>HPICEVSKVASHLEVNCDKRNLTALPPDLPKDTTILHLSENLLYTFSLATLMPYTRLTQLNLDRAELTKLQVDGTLPVLGTLDLSHNQLQSLPLLGQTLPALTVLDVSFNRLTSLPLGALRGLGELQELYLKGNELKTLPPGLLTPTPKLEKLSLANNNLTELPAGLLNGLENLDTLLLQENSLYTIPKGFFGSHLLPFAFLHGNPWLCNCEILYFRRWLQDNAENVYVWKQGVDVKAMTSNVASVQCDNSDKFPVYKYPGKGCPTLGDEGDTDLYDYYPEEDTEGDKVR[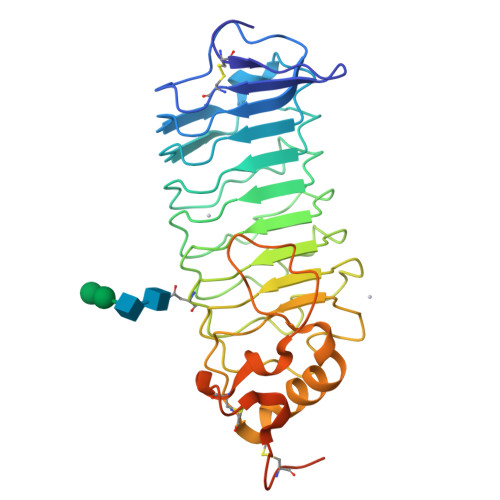2x]>[4x]MSTAIVTNVKHFGGMGSALRLSEAGHTVACHDESFKQKDELEAFAETYPQLKPM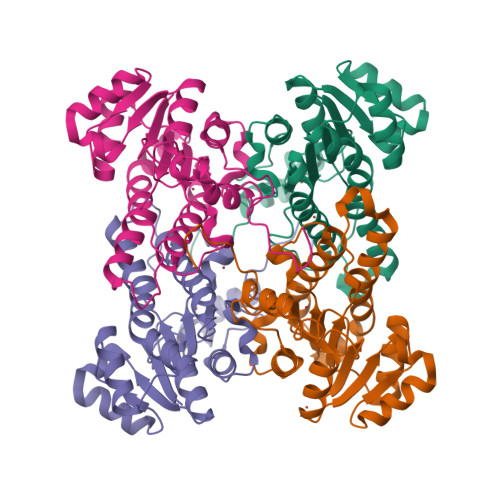SEQEPAELIEAVTSAYGQVDVLVSNDIFAPEFQPIDKYAVEDYRGAVEALQIRPFALVNAVASQMKKRKSGHIIFITSATPFGPWKELSTYTSARAGACTLANALSKELGEYNIPVFAIGPNYLHSEDSPYFYPTEPWKTNPEHVAHVKKVTALQRLGTQKELGELVAFLASGSCDYLTGQVFWLAGGFPMIERWPGMPE>[2x]MQYFSPEQQYNAWIVSDLVKQIFHKRAGCSPGIHELAVFAEEHFHIDIDFVFSIIMNIGDIEFALTDEIEKKLSGYLSTLLPYVTADMFETSKANAHAFLSRRHGNAAYHLFVSDDAFM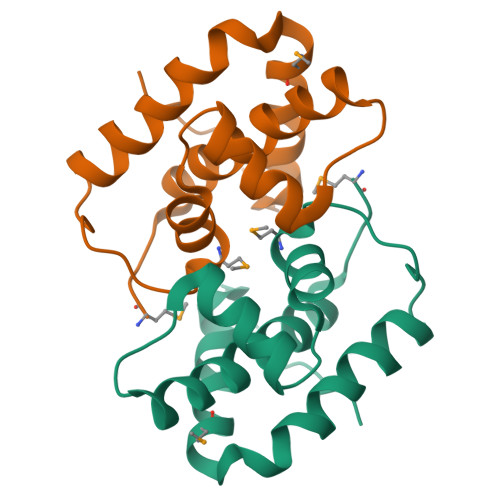RKQLEHHHHHH> MADDAIPHTDVLNSTAQG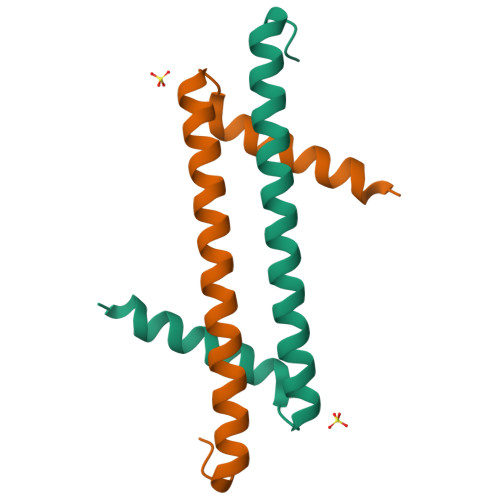QLKSIIERVERLEVEKAEIMEQIKEVYAEAKGNGFDVKVLKKVVRIRKQDRAKRLEHHHHHH>AGAIENARKEIKRISLEDHAESEYGAIYSVSGPVVIAENMIGCAMYELVKVGHDNLVGEVIRIDGDKATIQVYEETAGLTVGDPVLRTGKPLSVELGPGLMETIYDGIQRPLKAIKEESQSIYIPRGIDTPALDRTIKWQFTPGKFQVGDHISGGDIYGSVFENSLISSHKILLPPRSRGTITWIAPAGEYTLDEKILEVEFDGKKSDFTLYHTWPVRVPRPVTEKLSADYPLLTGQRVLDALFPCVQGGTTCIPGAFGCGKTVISQSLSKYSNSDAIIYVGCGERGNEMAEVLMEFPELYTEMSGTKEPIMKRTTLVANTSNMPVAAREASIYTGITLAEYFRDQGKNVSMIADSSSRWAEALREISGRLGEMPADQGFPAYLGAKLASFYERAGKAVALGSPDRTGSVSIVAAVSPAGGDFSDPVTTATLGITQVFWGLDKKLAQRKHFPSINTSVSYSKYTNVLNKFYDSNYPEFPVLRDRMKEILSNAEELEQVVQLVGKSALSDSDKITLDVATLIKEDFLQQNGYSTYDAFCPIWKTFDMMRAFISYHDEAQKAVANGANWSKLADSTGDVKHAVSSSKFFEPSRGEKEVHGEFEKLLSTMQERFAESTD[3x];>[3x]MVLSDKELFAINKKAVEQGFNVKPRLNYNTVSGVNGPLVILEKVKFPRYNEIVNLTLPDGTVRQGQVLEIRGDRAIVQVFEGTSGIDVKKTTVEFTGESLRIPVSEDMLGRIFDGSGRPIDNGPKVFAEDYLDINGSPINPYARIYPEEMISTGVSAIDTMNSIARGQKIPIFSASGLPHNEIAAQICRQAGLVRPTKDVHDGHEENFSIVFAAMGVNLETARFFKQDFEENGSLERTSLFLNLANDPTIERIITPRLALTTAEYLAYQTERHVLTILTDMSSYADALREVSAAREEVPGRRGYPGYMYTDLSTIYERAGRVEGRNGSITQIPILTMPNDDITHPIPDLTGYITEGQIFVDRQLHNKGIYPPINVLPSLSRLMKSAIGEGMTRKDHGDVSNQLYAKYAIGKDAAAMKAVVGEEALSIEDKLSLEFLEKFEKTFITQGAYEDRTVFESLDQAWSLLRIYPKEMLNRISPKILDEFYDRARDDADEDEEDPDTRSSGKKKDASQEESLI;>[3x]MSSAITALTPNQVNDELNKMQAFIRKEAEEKAKEIQLKADQEYEIEKTNIVRNETNNIDGNFKSKLKKAMLSQQITKSTIANKMRLKVLSAREQSLDGIFEETKEKLSGIANNRDEYKPILQSLIVEALLKLLEPKAIVKALERDVDLIESMKDDIMREYGEKAQRAPLEEIVISNDYLNKDLVSGGVVVSNASDKIEINNTLEERLKLLSEEALPAIRLELYGPSKTRKFFD;>MSQKNGIATLLQAEKEAHEIVSKARKYRQDKLKQAKTDAAKEIDSYKIQKDKELKEFEQKNAGGVGELEKKAEAGVQGELAEIKKIAEKKKDDVVKILIETVIKPSAEVHINAL[3x];> MSGNREQVFPTRMTLGLMKTKLKGANQGYSLLKRKSEALTKRFRDITKRIDDAKQKMGRVMQTAAFSLAEVSYATGENIGYQVQESVSTARFKVRARQENVSGVYLSQFESYIDPEINDFRLTGLGRGGQQVQRAKEIYSRAVETLVELASLQTAFIILDEVIKVTNRRVNAIEHVIIPRTENTIAYINSELDELDREEFYRLKKVQEKKQNETAKLDAEMKLKRDRAEQDASEVAADEEPQGETLVADQEDDVIF;> MAEKRTLIAVIADEDTTTGLLLAGIGQITPETQEKNFFVYQEGKTTKEEITDKFNHFTEERDDIAILLINQHIAENIRARVDSFTNAFPAILEIPSKDHPYDPEKDSVLKRVRKLFGE;> MATALYTANDFILISLPQNAQPVTAPGSKTDSWFNETLIGGRAFVSDFKIPEFKIGSLDTLIVESEELSKVDNQIGASIGKIIEILQGLNETSTNAYRTLPINNMPVPEYLENFQWQTRKFKLDKSIKDLITLISNESSQLDADVRATYANYNSAKTNLAAAERKKTGDLSVRSLHDIVKPEDFVLNSEHLTTVLVAVPKSLKSDFEKSYETLSKNVVPASASVIAEDAEYVLFNVHLFKKNVQEFTTAAREKKFIPREFNYSEELIDQLKKEHDSAASLEQSLRVQLVRLAKTAYVDVFINWFHIKALRVYVESVLRYGLPPHFNIKIIAVPPKNLSKCKSELIDAFGFLGGNAFMKDKKGKINKQDTSLHQYASLVDTEYEPFVMYIINL;> MGATKILMDSTHFNEIRSIIRSRSVAWDALARSEELSEIDASTAKALESILVKKNIGDGLSSSNNAHSGFKVNGKTLIPLIHLLSTSDNEDCKKSVQNLIAELLSSDKYGDDTVKFFQEDPKQLEQLFDVSLKGDFQTVLISGFNVVSLLVQNGLHNVKLVEKLLKNNNLINILQNIEQMDTCYVCIRLLQELAVIPEYRDVIWLHEKKFMPTLFKILQRATDSQLATRIVATNSNHLGIQLQYHSLLLIWLLTFNPVFANELVQKYLSDFLDLLKLVKITIKEKVSRLCISIILQCCSTRVKQHKKVIKQLLLLGNALPTVQSLSERKYSDEELRQDISNLKEILENEYQELTSFDEYVAELDSKLLCWSPPHVDNGFWSDNIDEFKKDNYKIFRQLIELLQAKVRNGDVNAKQEKIIIQVALNDITHVVELLPESIDVLDKTGGKADIMELLNHSDSRVKYEALKATQAIIGYTFK;> MEGVYFNIDNGFIEGVVRGYRNGLLSNNQYINLTQCDTLEDLKLQLSSTDYGNFLSSVSSESLTTSLIQEYASSKLYHEFNYIRDQSSGSTRKFMDYITYGYMIDNVALMITGTIHDRDKGEILQRCHPLGWFDTLPTLSVATDLESLYETVLVDTPLAPYFKNCFDTAEELDDMNIEIIRNKLYKAYLEDFYNFVTEEIPEPAKECMQTLLGFEADRRSINIALNSLQSSDIDPDLKSDLLPNIGKLYPLATFHLAQAQDFEGVRAALANVYEYRGFLETGNLEDHFYQLEMELCRDAFTQQFAISTVWAWMKSKEQEVRNITWIAECIAQNQRERINNYISVY;>MTELCPVYAPFFGAIGCASAIIFTSLGAAYGTAKSGVGICATCVLRPDLLFKNIVPVIMAGIIAIYGLVVSVLVCYSLGQKQALYTGFIQLGAGLSVGLSGLAAGFAIGIVGDAGVRGSSQQPRLFVGMILILIFAEVLGLYGLIVALLLNSRATQDVVC[10x];> MAEKEEAIFRSAEMALVQFYIPQEISRDSAYTLGQLGLVQFRDLNSKVRAFQRTFVNEIRRLDNVERQYRYFYSLLKKHDIKLYEGDTDKYLDGSGELYVPPSGSVIDDYVRNASYLEERLIQMEDATDQIEVQKNDLEQYRFILQSGDEFFLKGDNTDSTSYMDEDMIDANGENIAAAIGASVNYVTGVIARDKVATLEQILWRVLRGNLFFKTVEIEQPVYDVKTREYKHKNAFIVFSHGDLIIKRIRKIAESLDANLYDVDSSNEGRSQQLAKVNKNLSDLYTVLKTTSTTLESELYAIAKELDSWFQDVTREKAIFEILNKSNYDTNRKILIAEGWIPRDELATLQARLGEMIARLGIDVPSIIQVLDTNHTPPTFHRTNKFTAGFQSICDCYGIAQYREINAGLPTIVTFPFMFAIMFGDMGHGFLMTLAALSLVLNEKKINKMKRGEIFDMAFTGRYIILLMGVFSMYTGFLYNDIFSKTMTIFKSGWKWPDHWKKGESITATSVGTYPIGLDWAWHGTENALLFSNSYKMKLSILMGFIH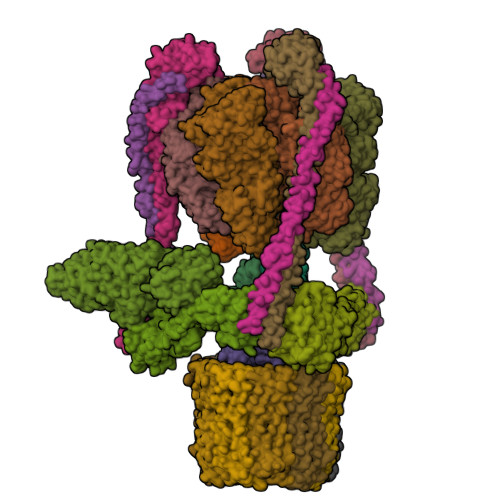MTYSYFFSLANHLYFNSMIDIIGNFIPGLLFMQGIFGYLSVCIVYKWAVDWVKDGKPAPGLLNMLINMFLSPGTIDDELYPHQAKVQVFLLLMALVCIPWLLLVKPLHFKFTHKKKSHEPLPSTEADASSEDLEAQQLISAMDADDAEEEEVGSGSHGEDFGDIMIHQVIHTIEFCLNCVSHTASYLRLWALSLAHAQLSSVLWTMTIQIAFGFRGFVGVFMTVALFAMWFALTCAVLVLMEGTSAMLHSLRLHWVESMSKFFVGEGLPYEPFAFEYKDMEVAVASASSSASS>[2x]MDVKHIAKQTTKTLISYLTYQAVRTVIGQLAETDPPRSLWLHQFTSQESIQDGER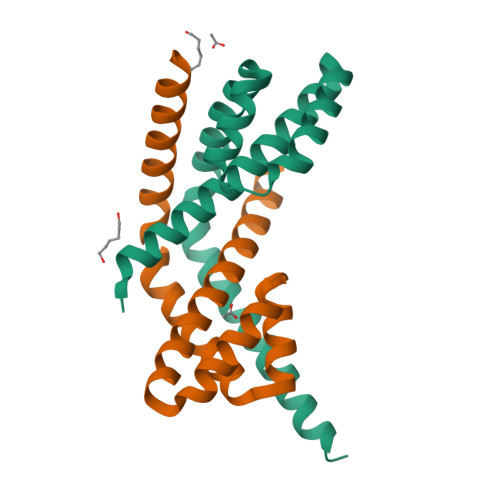YLEALFREQPDLGFRILTVREHLAEMVADYLPEMLRAGIQQANLQQRAQQLERMTQVSEANVENSNLETPE> GPGSEFRPLPPGWEKRTDPRGRFYYVDHNTRTTTWQRPTAEYVRNYEQWQSQRNQLQGAMQHFSQRFLYQSSSASTDHDPLGPENLYFQGESGTKQGSPGAYDRSFRWKYHQFRFLCHSNALPSHVKISVSRQTLFEDSFQQIMNMKPYDLRRRLYIIMRGEEGLDYGGIAREWFFLLSHEVLNPMYCLFEYAGKNNYCLQINPASSINPDHLTYFRFIGRFIAMALYHGKFIDTGFTLPFYKRMLNKRPTLKD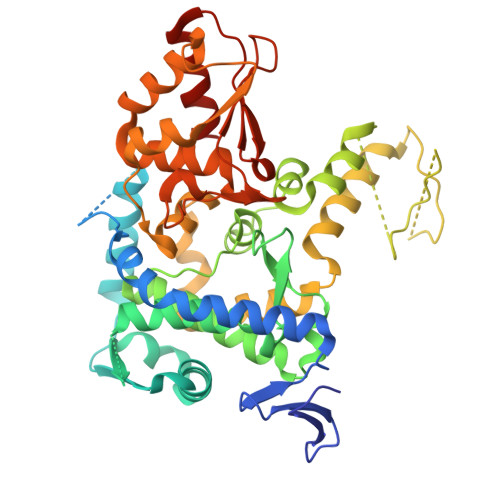LESIDPEFYNSIVWIKENNLEECGLELYFIQDMEILGKVTTHELKEGGESIRVTEENKEEYIMLLTDWRFTRGVEEQTKAFLDGFNEVAPLEWLRYFDEKELELMLCGMQEIDMSDWQKSTIYRHYTKNSKQIQWFWQVVKEMDNEKRIRLLQFVTGTCRLPVGGFAELIGSNGPQKFCIDKVGKETWLPRSHTCFNRLDLPPYKSYEQLREKLLYAIEETEGFGQE>[2x]MTVRKNQATLTADEKRRFVAAVLELKRSGRYDEFVRTHNEFIMSDTDSGERTGHRSPSFLPWHRRFLLDFEQALQSVDSSVTLPYWDWSADRTVRASLWAPDFLGGTGRSTDGRVMDGPFAASTGNWPINVRVDSRTYLRRSLGGSVAELPTRAEVESVLAI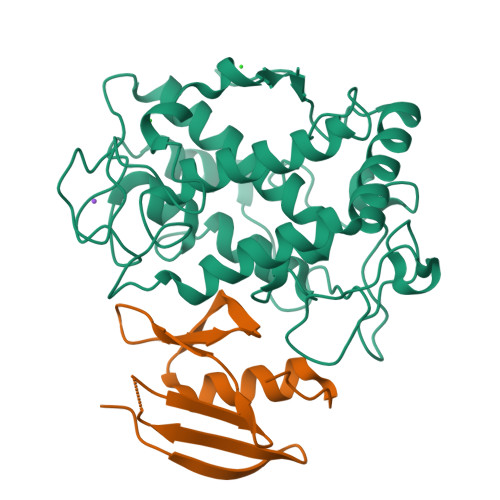SAYDLPPYNSASEGFRNHLEGWRGVNLHNRVHVWVGGQMATGVSPNDPVFWLHHAYVDKLWAEWQRRHPDSAYVPTGGTPDVVDLNETMKPWNTVRPADLLDHTAYYTFDALEHHHHHH;>MPEITRRRALTAAAAVAATASAAVTLAAPAASAAGHHEPAAPESFDEVYKGRRIQGRPARGAAHHHEHGGGYEVFVDGVQLHVMRNADGSWISVVSHYDPVPTPRAAARAAVDELQGAPLLPFPANLEHHHHHH[2x]>MTLSPEKQHVRPRDAADNDPVAVARGLAEKWRATAVERDRAGGSATAEREDLRASGLLSLLVPREYGGWGADWPTAIEVVREIAAADGSLGHLFGYHLTNAPMIELIGSQEQEEHLYTQIAQNNWWTGNASSENNSHVLDWKVRATPTEDGGYVLNGTKHFCSGAKGSDLLFVFGVVQDDSPQQGAIIAAAIPTSRAGVTPNDDWAAIGMRQTDSGSTDFHNVKVEPDEVLGAPNAFVLAFIQSERGSLFAPIAQLIFANVYLGIAHGALDAAREYTRTQARPWTPAGIQQATEDPYTIRSYGEFTIALQGADAAAREAAHLLQTVWDKGDALTPEDRGELMVKVSGVKALATNAALNISSGVFEVIGARGTHPRYGFDRFWRNVR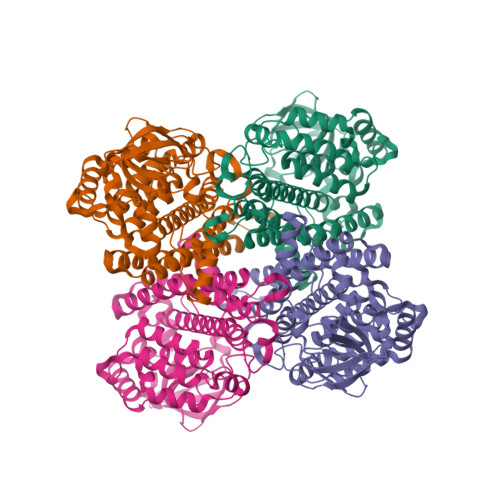THSLHDPVSYKIADVGKHTLNGQYPIPGFTS[8x]3,3-difluorocyclobutyl {(2R,4S,6S,12Z,13aS,14aR,16aS)-2-[(7-methoxy-3-methylquinoxalin-2-yl)oxy]-14a-[(1-methylcyclopropane-1-sulfonyl)carbamoyl]-5,16-dioxo-1,2,3,5,6,7,8,9,10,11,13a,14,14a,15,16,16a-hexadecahydrocyclopropa[e]pyrrolo[1,2-a][1,4]diazacyclopentadecin-6-yl}carbamate 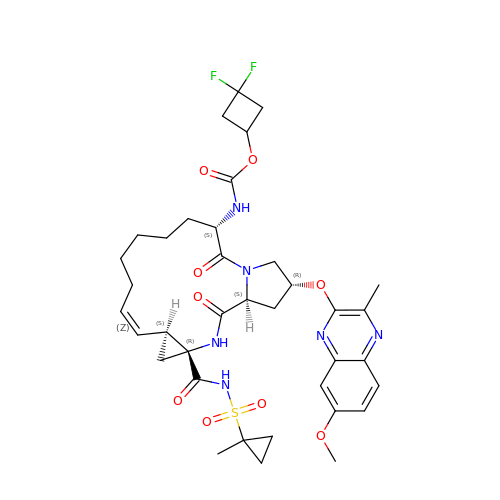| C37 H46 F2 N6 O9 S | GNPRLAOVQQDDAJ-SKXVKYEHSA-N>MPPYTVVYFPVRGRCAALRMLLADQGQSWKEEVVTVETWQEGSLKASCLYGQLPAFQDGDLTLYQSNTILRHLGRTLGLYGKDQQEAALVDMVNDGVEDLRCKYISLIYTNYEAGKDDYVKALPGQLKPFETLLSQ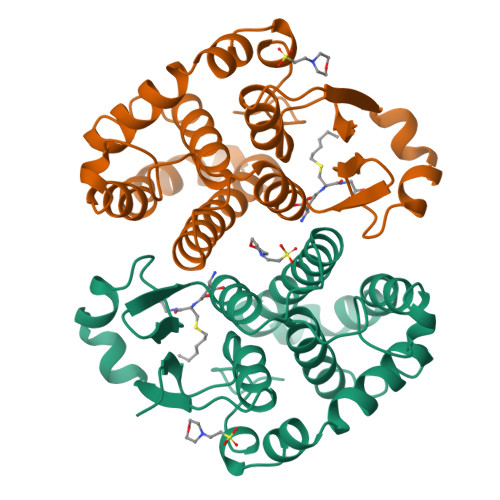NQGGKTFIVGDQISFADYNLLDLLLIHEVLAPGCLDAFPLLSAYVGRLSARPKLKAFLASPEYVNLPINGNGKQ[2x]>[20x]SMKINAENFECLRESKLKRKVYEDLVKEATFVRVSPKSTVCVVTDHNSFEVIGTSSVYKVENFNDEIGRDTALSQALDSFIKFLAYSGELSDVLENI

In this study, we discover Acb4 from the Bacillus phage SPO1 as the founding member of a widespread family of >1,300 anti-CBASS immune evasion proteins. We demonstrate that Acb4 is a phage-encoded sponge that sequesters CBASS signals to subvert host anti-phage defense, highlighting viral inhibition of host nucleotide immune signals as a conserved mechanism of immune evasion. CBASS operons encode two main components: a cGAS/DncV-like nucleotidyltransferase (CD-NTase) enzyme that responds to phage infection and catalyzes the synthesis of a nucleotide immune signal, and a CD-NTase-associated protein (Cap) effector that recognizes the nucleotide immune signal and induces cell death or cell stasis to prevent phage propagation. Acb4 is a small 96 amino acid protein that assembles into a tetrameric pinwheel-like structure.

To define the molecular mechanism of Acb4 nucleotide sequestration and CBASS evasion, we determined a 2.10 Å crystal structure of the phage SPO1 Acb4–3′3′-cGAMP complex (Crystallographic Statistics). Each Acb4 protomer is composed of a core region of three antiparallel β-strands (β1–β3) flanked by an N-terminal helical region (α1–α3) and a longer C-terminal extension with two helices (α4–α5). Individual Acb4 protomers form two distinct protein–protein interfaces that interlock to create the tetrameric pinwheel-like assembly. The Acb4 3′3′-cGAMP-binding site is situated in a pocket formed between an extended β3–α4 loop region of one protomer and helices α4 and α5 from the opposite dimeric unit. 3′3′-cGAMP ligands bind within each of the four equivalent interfaces creating a 4:4 Acb4–3′3′-cGAMP assembly. The 3′3′-cGAMP ligand binding site is formed at the interface between two partnering protomers (denoted Acb4A and Acb4B) and a third protomer from the opposite dimeric unit (Acb4C). Notably, the phage SPO1 Acb4A–Acb4B interface creates distinct adenine and guanine nucleobase pockets that allow sequence-specific recognition of 3′3′-cGAMP. Recognition of guanine occurs through Acb4 residues K36A and E49B that coordinate sequence-specific contacts with the nucleobase Watson-Crick edge. In the opposite pocket, adenine recognition occurs through peptide backbone interactions between Acb4 residue N63A and the adenine Watson-Crick edge, and an additional network of van der Waals contacts formed by residues V56A, F62A, and I66A that sterically restrict access of guanine nucleobases. Contacts between Acb4 residues Y57A, T70A, and K81C and the diphosphate backbone of 3′3′-cGAMP further stabilize ligand recognition.> MLYLTQRLEIPAAATASVTLPIDVRVKSRVKVTLNDGRDAGLLLPRGLLLRGGDVLSNEEGTEFVQVIAADEEVSVVRCDDPFMLAKACYALGNRHVPLQI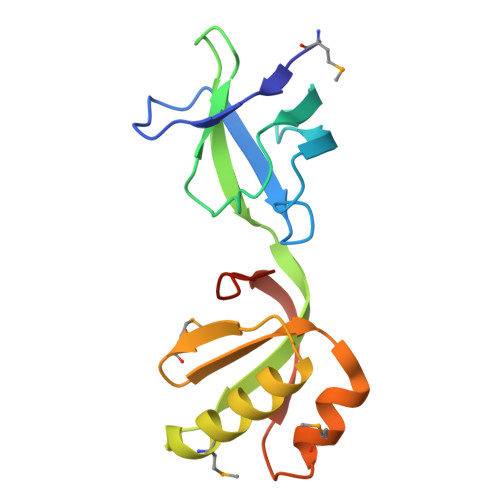MPGELRYHHDHVLDDMLRQFGLTVTFGQLPFEPEAGAYASES>MTTHNSQYSAETTHPDKQESSPAPTAAGTTASNVSTTGNATTPDASIALNADATPVADVPPRLFGSFVEHLGRCVYGGIYEPSHPTADENGFRQDVLDLVKELGVTCVRYPGGNFVSNYNWEDGIGPRENRPMRRDLAWHCTETNEMGIDDFYRWSQKAGTEIMLAVNMGTRGLKAALDELEYVNGAPGTAWADQRVANGIEEPMDIKMWCIGNEMDGPWQVGHMSPEEYAGAVDKVAHAMKLAESGLELVACGSSGAYMPTFGTWEKTVLTKAYENLDFVSCHAYYFDRGHKTRAAASMQDFLASSEDMTKFIATVSDAADQAREANNGTKDIALSFDEWGVWYSDKWNEQEDQWKAEAAQGLHHEPWPKSPHLLEDIYTAADAVVEGSLMITLLKHCDRVRSASRAQLVNVIAPIMAEEHGPAWRQTTFYPFAEAALHARGQAYAPAISSPTIHTEAYGDVPAIDAVVTWDEQARTGLLLAVNRDANTPHTLTIDLSGLPGLPGLGTLALGKAQLLHEDDPYRTNTA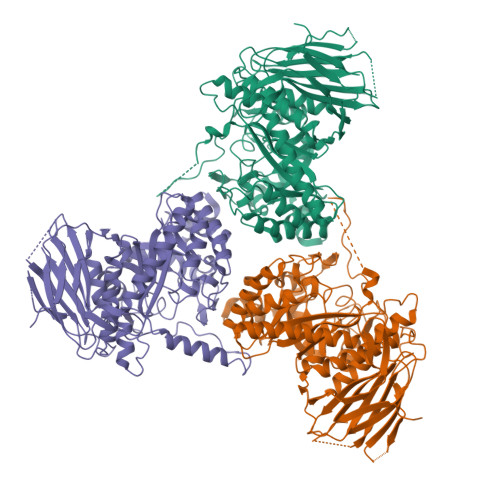EAPEAVTPQPLDIAMNATGTCTATLPAISWISVEFHGKGHHHHHH[6x]2-(4-ISOPROPYL-4-METHYL-5-OXO-4,5-DIHYDRO-1H-IMIDAZOL-2-YL)QUINOLINE-3-CARBOXYLIC ACID | C17 H17 N3 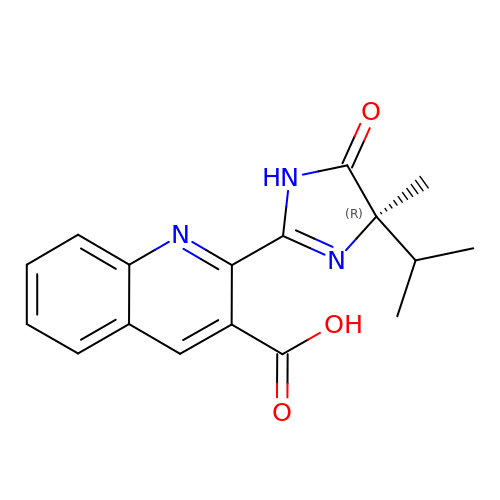O3 | CABMTIJINOIHOD-QGZVFWFLSA-N>MSYQHPWCARLLTSLPDEQIRGAVLADEPRWDYVETELVKLGSLAHSQVDLNAVAEACLGLLESRTKDMRVLAQLLRCLQHPAKATPLGAAISLLEAWIQAYWLLAWPGNASQKQRLMVQIVKRFEGALPRICESASAAELAQLLAQAEQLERVWLAQCPDKGELLDPLVMGLKRAQRQQLAQAEANAAGQPQSSGAAAAGSPASVASTASCAGAMVLSGSAGVDVDSSNDRAWRQTQLKVAELLIERQPEVAVGYRLRRHAVWAGITAVPMSGAGNKTPLAPMSADMVDEYRAAMNAPDQGLWQRIEQSLTLAPYWFEGHRLSAEVAEKLGFGAVAQAIAEELGTFLQRLPALRELAFSDGSPFLSPECSRWLLEHH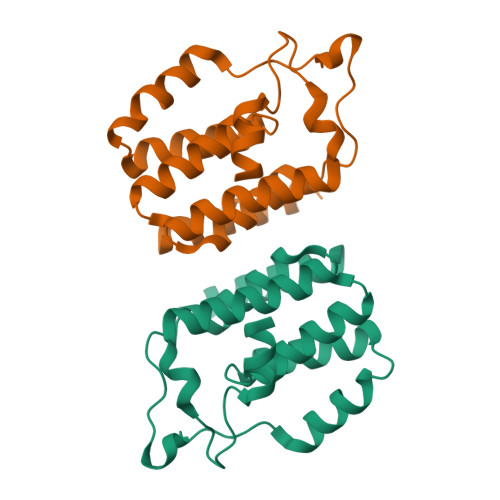HHHH[4x]>[6x]MKFSKEQFDYSLYLVTDSGMIPEGKTLYGQVEAGLQNGVTLVQIREKDADTKFFIEEALQIKELCHAHNVPLIINDRIDVAMAIGADGIHVGQDDMPIPMIRKLVGPDMVIGWSVGFPEEVDELSKMGPDMVDYIGVGTLFPTLTKKNPKKAPMGTAGAIRVLDALERNNAHWCRTVGIGGLHPDNIERVLYQCVSSNGKRSLDGICVVSDIIASLDAAKSTKILRGLIDKTDYKFVNIGLSTKNSLTTTDEIQSIISNTLKARPLVQHITNKVHQNFGANVTLALGSSPIMSEIQSEVNDLAAIPHATLLLNTGSVAPPEMLKAAIRAYNDVKRPIVFDPVGYSATETRLLLNNLLLTFGQF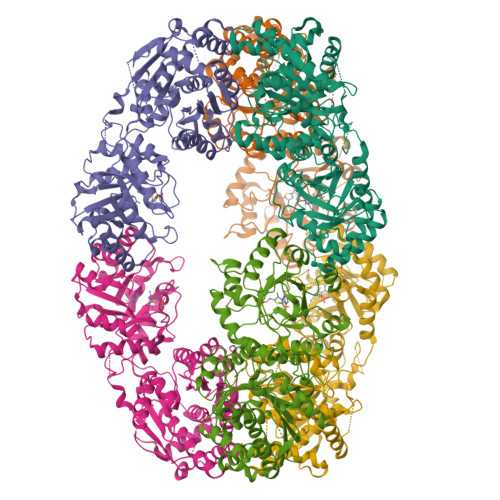SCIKGNSSEILGLAELNKERMKGVDASSGISNELLIQATKIVAFKYKTVAVCTGEFDFIADGTIEGKYSLSKGTNGTSVEDIPCVAVEAGPIEIMGDITASGCSLGSTIACMIGGQPSEGNLFHAVVAGVMLYKAAGKIASEKCNGSGSFQVELIDALYRLTRENTPVTWAPKLTHT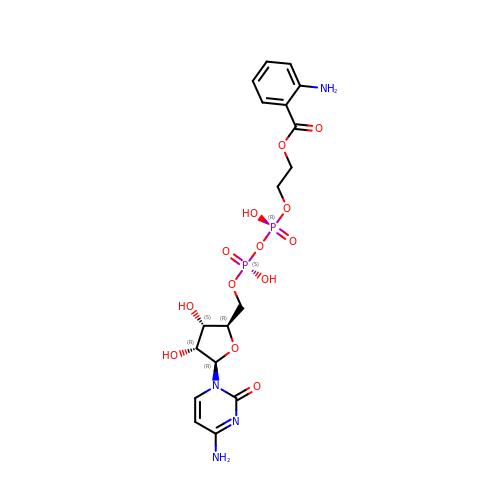5'-O-[({[(2-{[(2-AMINOPHENYL)CARBONYL]OXY}ETHYL)OXY]PHOSPHINATO}OXY)PHOSPHINATO]CYTIDINE | C18 H24 N4 O13 P2 | PGXVRIOOHRVKLC-DTZQCDIJSA-N> MGSSHHHHHHSSGRENLYFQGHMNGDQNSDVYAQEKQDFVQHFSQIVRVLTEDEMGHPEIGDAIARLKEVLEYNAIGGKYNRGLTVVVAFRELVEPRKQDADSLQRAWTVGWCVELLQAFFLVADDIMDSSLTRRGQICWYQKPGVGLDAINDANLLEACIYRLLKLYCREQPYYLNLIELFLQSSYQTEIGQTLDLLTAPQGNVDLVRFTEKRYKSIVKYKTAFYSFYLPIAAAMYMAGIDGEKEHANAKKILLEMGEFFQIQDDYLDLFGDPSVTGKIGTDIQDNKCSWLVVQCLQRATPEQYQILKENYGQKEAEKVARVKALYEELD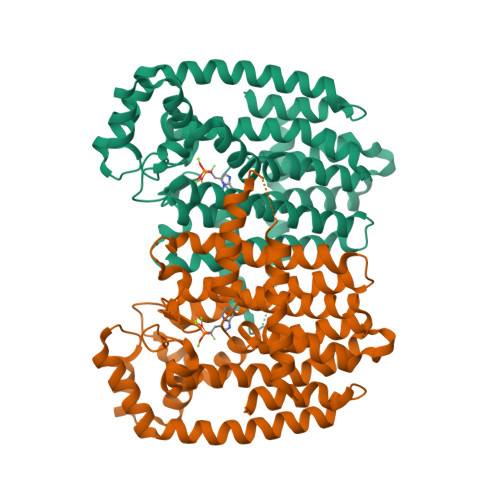LPAVFLQYEEDSYSHIMALIEQYAAPLPPAVFLGLARKIYKRRK>[2x]GMDV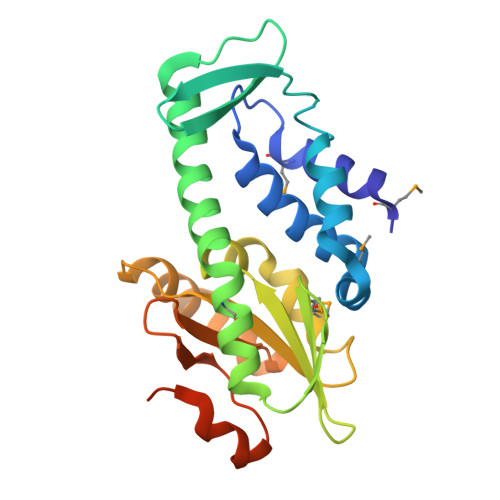EIVEELSKMLAGRKAVTEEEIRRKAIRCALKIMGARLVGIDAELIEDVTCSLIDCPITLKSLHFSEKVKIGDVLFYHPHVIKPEKEDFEQAYFEYKQSKKFLDAFDIMREVTDRFFEGYEAEGRYMRKYTKDGRNYYAFFSTIDDTFEDVDIHLRMVDEVDGDYVVIVPTENELNPFLKFFKQYSEDAKRAGLKIWVVNPDEKTIDPFIGYPKDFRLLKGFKNPKAAALVSAYWRVTVTDLD> GPGSVRVVRGRGLLRAVLDRPERRNPIDAGLLTSLARALDQAESDQDCRVFVLSSTGEDFCAGTDLSGGDPAPEPLPDGAELPYWTLLERLTRSPLATVAVVDGRATAGGVGLAAACDLVLAGERARFRLTEVLAGLVPAMALPFVARRTGEQRAFAATLRAEEFDAGAAHRVGLADLAGPR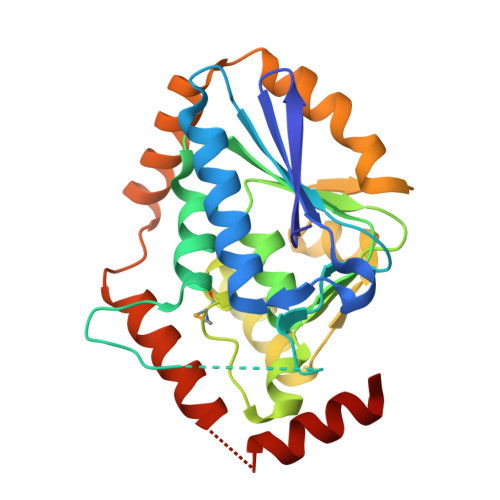AEDLLPPVLAGLGRTDRSTTAALKEYRARLFPRDARLGHDASRLLIERFAAPGTGQLLARLREAGAAA> MAIIETTTPTEEEAKAIAKKLLENRLIAEAIITPALTKIYRENGEIKSETVTRVTLYTEEENVPKAVTYIKAIHPDPIPPIIVITPTDAN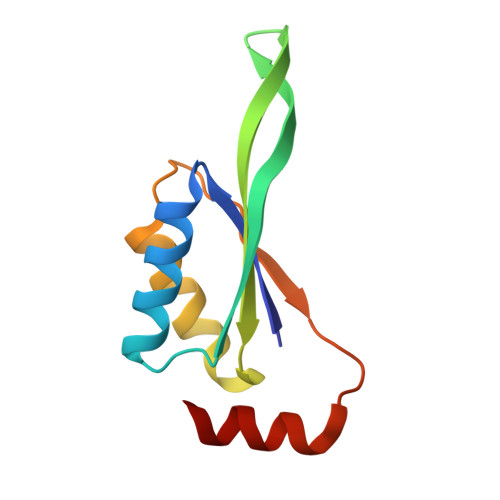PAYKGWVAFET> QFRAIIESPEGAGHVGYQYRRNTGSTMRMVSDVLDERVSLWDFHCDPSGNVIQPGPNVDSRQYLQAAIDYVSSNGGGTITIPAGYTWYLGSYGVGGIAGHSGIIQLRSNVNLNIEGRIHLSPFFDLKPFQVFVGFDNGDPASSGNLENCHIYGHGVVDFGGYEFGASSQLRNGVAFGRSYNCSVTGITFQNGDVTWAITLGWNGYGSNCYVRKCRFINLVNSSVNAAHSTVYVNCPYSGVESCYFSMSSSFARNIACSVELHQHDTFYRGSTVNGYCRGAYVVMHAAEAAGAGSYAYNMQVENNIAVIYGQFVILGSDVTATVSGHLNDVIVSGNIVSIGERAAFSAPFGAFIDIGPDNSGASNVQDIQRVLVTGNSFYAPANITDSAAITLRANLNGCTFIANNFDCRYMVYNAPGTTSPVVQNLV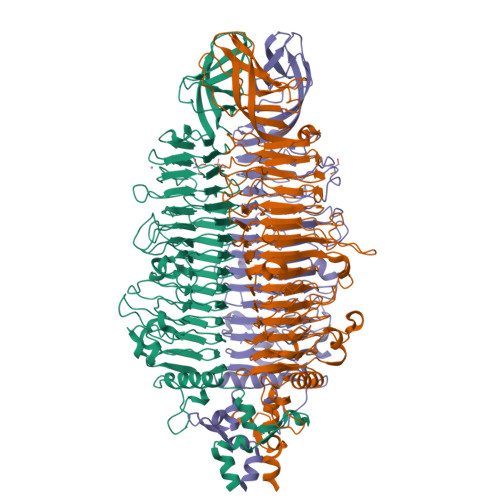WDKSNVIGGTHANQRAGQNLFDMQFASVVNSTIEVQLSCEDLSMFSCILFPASCQLSYSKITVDSAWTKSMSNTAVFEGNQQAGANVYVSYPATVNLTSYNTQGAVPFFSTDTNYAWVTSAYSLSINENLDFSPPATYTNKANGQLVGVGYNEIGGVRSVSVRLMLQRQV>[4x]MLRKLAAVSLLSLLSAXLLAAECSVDIQGNDQMQFNTNAITVDKSCKQFTVNLSHPGNLPKNVMGHNWVLSTAADMQGVVTDGMASGLDKDFLKPDDSR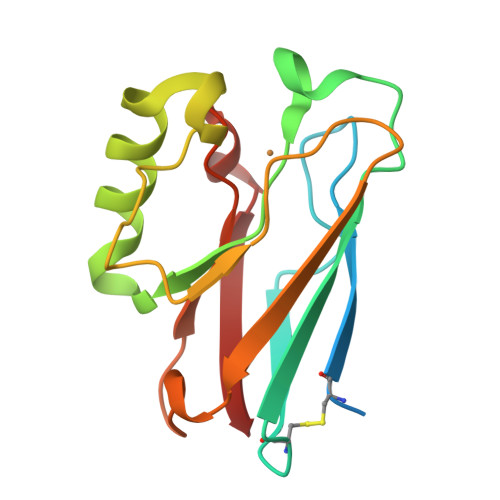VIAHTKLIGSGEKDSVTFDVSKLKEGEQFMAFCTFPGHSALMKGTLTLK> METTVSKLERQIEERLKGVSEYESININHRLGKLLDSYDIPDVAKVACLTIDTSMRHLDDITYNHLSKHSILIGDLISAHFYTLLAEINDLSFQNEISKAIVEINELKSSLHHQALNDYEISQAIVKIETLFPYITLSHFGINIDESEIYNYLFEDMSDYYPSYFKKYNQSEVKHYLH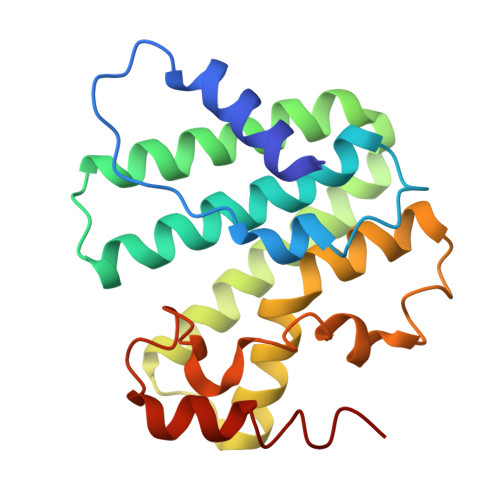DIQKSYLKSRGN>[3x]MKNDLIRPNVLSVKIISNVSPEMAKKLELEPHHKSLGLITADCDDVTYTALDEATKAAEVDVVYARS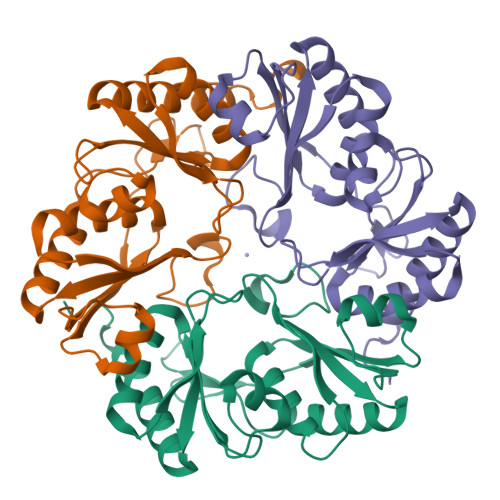MYAGAGNASTKLAGEVIGILAGPSPAEVRSGLNATLDFIDSGVGFVSANEDDSICYYAQCVSRTGSYLSKTAGIREGEALAYLVAPPLEAMYALDAALKAADVEMCEFFAPPTETNFAGALLTGSQSACKAACDAFAEAVQSVASNPLGFLEHHHHHH>[6x]MEQYSEACIEACIDCMKACNHCF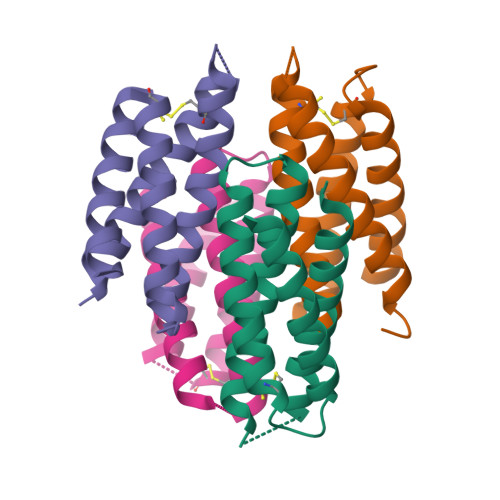TKCLEESVQHHLSGCIRLDRECADICALAVKAMQTDSPFMKEICALCADICEACGTECGKHDHDHCQACAKACFTCAEQCRSMAA> MSEAPKKRWYVVQAFSGFEGRVATSLREHIKLH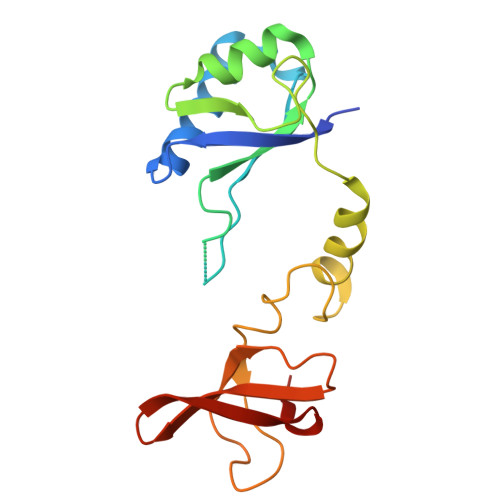NMEDLFGEVMVPTEEVVEIRGGQRRKSERKFFPGYVLVQMVMNDASWHLVRSVPRVMGFIGGTSDRPAPISDKEVDAIMNRLQQVGDKPRPKTLFEPGEMVRVNDGPFADFNGVVEEVDYEKSRLKVSVSIFGRATPVELDFSQVEKA> MTTYLEFIQQNEERDGVRFSWNVWPSSRLEATRMVVPVAALFTPLKERPDLPPIQYEPVLCSRTTCRAVLNPLCQVDYRAKLWACNFCYQRNQFPPSYAGISELNQPAELLPQFSSIEYVVLRGPQMPLIFLYVVDTCMEDEDLQALKESMQMSLSLLPPTALVGLITFGRMVQVHELGCEGISKSYVFRGTKDLSAKQLQEMLGLSKVPLTQATRGPQVQQPPPSNRFLQPVQKIDMNLTDLLGELQRDPWPVPQGKRPLRSSGVALSIAVGLLECTFPNTGARIMMFIGGPATQGPGMVVGDELKTPIRSWHDIDKDNAKYVKKGTKHFEALANRAATTGHVIDIYACALDQTGLLEMKCCPNLTGGYMVMGDSFNTSLFKQTFQRVFTKDMHGQFKMGFGGTLEIKTSREIKISGAIGPCVSLNSKGPCVSENEIGTGGTCQWKICGLSPTTTLAIYFEVVNQHNAPIPQGGRGAIQFVTQYQHSSGQRRIRVTTIARNWADAQTQIQNIAASFDQEAAAILMARLAIYRAETEEGPDVLRWLDRQLIRLCQKFGEYHKDDPSSFRFSETFSLYPQFMFHLRRSSFLQVFNNSPDESSYYRHHFMRQDLTQSLIMIQPILYAYSFSGPPEPVLLDSSSILADRILLMDTFFQILIYHGETIAQWRKSGYQDMPEYENFRHLLQAPVDDAQEILHSRFPMPRYIDTEHGGSQARFLLSKVNPSQTHNNMYAWGQESGAPILTDDVSLQVFMDHLKKLAVSSAA;> SPIQVIENDRASRGGQVYATNTRGQIPPLVTTDCMIQDQGNASPRFIRCTTYCFPCTSDMAKQAQIPLAAVIKPFATIPSNESPLYLVNHGESGPVRCNRCKAYMCPFMQFIEGGRRYQCGFCNCVNDVPPFYFQHLDHIGRRLDHYEKPELSLGSYEYVATLDYCRKSKP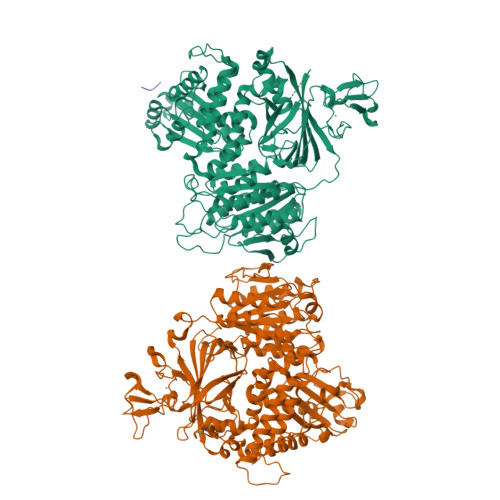PNPPAFIFMIDVSYSNIKNGLVKLICEELKTMLEKIPKEEQEETSAIRVGFITYNKVLHFFNVKSNLAQPQMMVVTDVGEVFVPLLDGFLVNYQESQSVIHNLLDQIPDMFADSNENETVFAPVIQAGMEALKAADCPGKLFIFHSSLPTAEAPGKLKNRDDKKLVNTDKEKILFQPQTNVYDSLAKDCVAHGCSVTLFLFPSQYVDVASLGLVPQLTGGTLYKYNNFQMHLDRQQFLNDLRNDIEKKIGFDAIMRVRTSTGFRATDFFGGILMNNTTDVEMAAIDCDKAVTVEFKHDDKLSEDSGALIQCAVLYTTISGQRRLRIHNLGLNCSSQLADLYKSCETDALINFFAKSAFKAVLHQPLKVIREILVNQTAHMLACYRKNCASPSAASQLILPDSMKVLPVYMNCLLKNCVLLSRPEISTDERAYQRQLVMTMGVADSQLFFYPQLLPIHTLDVKSTMLPAAVRCSESRLSEEGIFLLANGLHMFLWLGVSSPPELIQGIFNVPSFAHINTDMTLLPEVGNPYSQQLRMIMGIIQQKRPYSMKLTIVKQREQPEMVFRQFLVEDKGLYGGSSYVDFLCCVHKEICQLLN;> GPRPLPPP>RPPQFTRAQWFAIQHISLNPPRCTIAMRAINNYRWRCKNQNTFLRTTFANVVNVCGNQSIRCPHNRTLNNCHRSRFRVPLLHCDLINPGAQNIS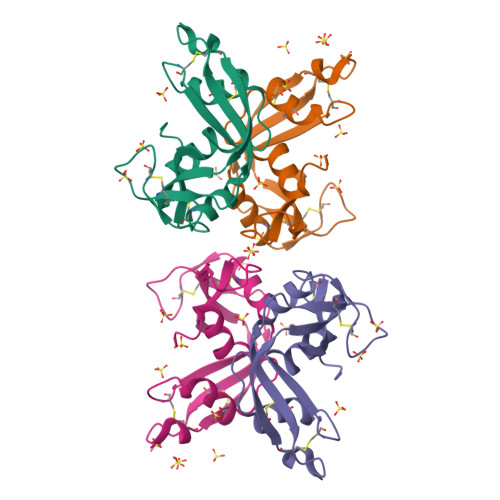NCRYADRPGRRFYVVACDNRDPRDSPRYPVVPVHLDTTI[2x]>MRGSHHHHHHGSMDKNIIIGAMTALITPFKNGKVDEQSYARLIKRQIENGIDAVVPVGTTGESATLTHEEKRTCIEIAVETCKGTKVKVLAGAGSNATHEAVGLAKFAKEHGADGILSVAPYYNKPTQQGLYEHYKAIAQSVDIPVLLYNVPGRTGCEISTDTIIKLFRDCENIYGVKEASGNIDKCVDLLAHEPRMMLISGEDAINYPILSNGGKGVISVTSNLLPDMISALTHFALDENYKEAKKINDELYNINKILFCESNPIPIKTAMYL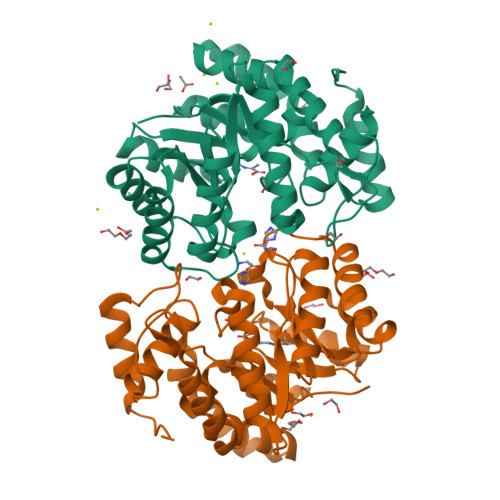AGLIESLEFRLPLCSPSKENFAKIEEVMKKYKIKGF[6x]>MLVSVYLALLVACVGQAHSQANLMRLKSDLFNRSPMYPGPTKDDPLTVTLGFFLQDIVKVDSSTNEVDLVYYERQRWKLNSLMWDPNEYGNITDFRTSAADIWTPDITAASSTRPVQVLSPQIAVVTHDGSVMF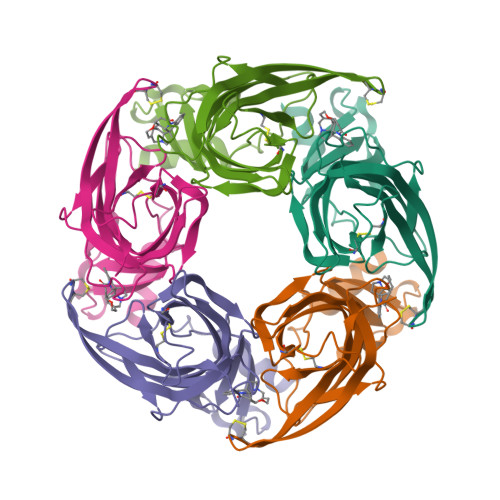SPAQRLSFMCDPTGVDSEEGVTCAVKFESWVYSGFEIDLKTDTDQVDLSSYYASSKYEILSATQTRQVQHYSCCPEPYIDVNLVVKFRERRAGNGFFRNLFDENLYFQGHHHHHH[15x]> MSNLSGTDKSVILLMTIGEDRAAEVFKHLSTREVQALSTAMANVRQISNKQLTDVLSEFEQEAEQFAALNINANEYLRSVLVKALGEERASSLLEDILETRDTTSGIETLNFMEPQSAADLIRDEHPQIIATILVHLKRSQAADILALFDERLRHDVMLRIATFGGVQPAALAELTEVLNGLLDGQNLKRSKMGGVRTAAEIINLMKTQQEEAVITAVR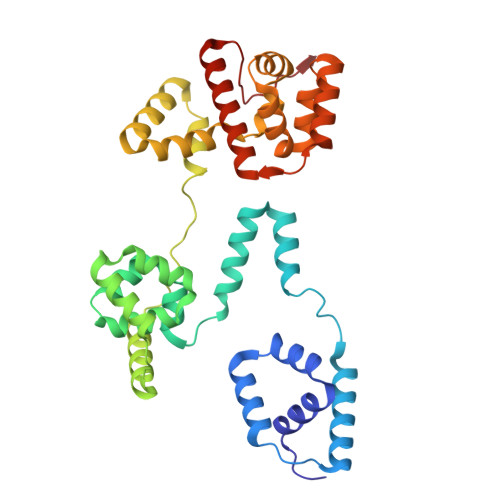EFDGELAQKIIDEMFLFENLVDVDDRSIQRLLQEVDSESLLIALKGAEPPLREKFLRNMSQRAADILRDDLANRGPVRLSQVENEQKAILLIVRRLAETGEMVIGSGEDTYV> KDHQLLR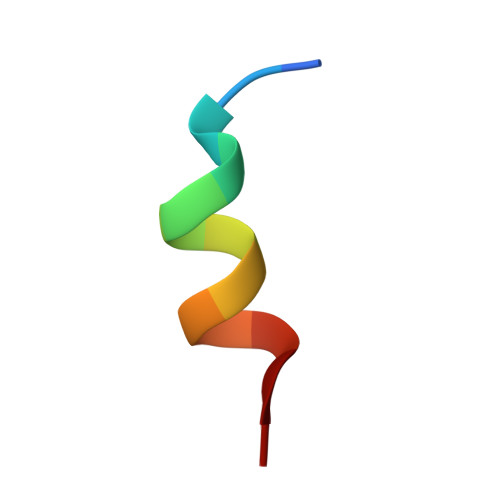YLLDKD>MAHHHHHHVGTFENITAAPADPILGLADLFRADERPGKVDLGVGVYKDETGKTPVLTSVKKAEQYLLENETTKTYLGLDGLPEFGRCTQELLFGKGSALINDKRARTAQTPGGSGALRVAADFLAKNTSVKRVWVSNPSWPNHKAIFNSAGLEVREYAYYDAENHTLDFDALINSLNEAQAGDVVLFHGCCHNPTGADPTLEQWQTLAQLSVEKGWLPLIDIAYQGFGRGLEEDAEGLRAFAAMHKELIVASSCSKNFGLYNERVGACTLVAADSETVDRAFSQMKAAIRANYSNPPAHGASVVATILSNDALRAIWEQELTDMRQRIQRMRQLFVNTLQEKGANRDFSFIIKQNGMFSFSGLTKEQVLRLREEFGVYAVASGRVNVAGMTP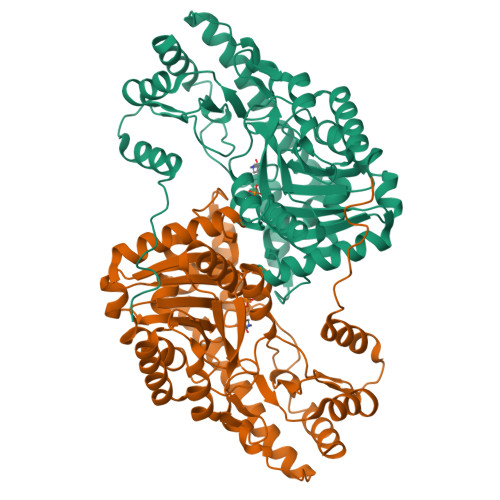DNMAPLCEAIVAVL[2x]>[4x]HHHHHHMALQLAAHSDARSGPVGSNGGQFWSFRPVRPLNKIVLSFSGSPDQTLNLISITFSSNPTDIITVGGVGPEPLTYTETVNIDGDIIEISGMIANYKGYNVIRSIKFTTNKKEYGPYGANAGTPFNIKIPDGNKIVGFFGNSGWYVDAIGAYYTAK

Structural and functional analysis identified IPO as a member of the JRL family but with a different tetrameric association. The monomeric IPO from residues 1 to 154 shows a typical β-prism fold found in the JRL family, with 12 β-sheets (β3-β14) and 2 additional short, extended, N-terminal β-strands (β1-β2). Four IPO protomers form a compact tetrameric association by swapping their extended N termini from residues 1 to 10. Thus, the wound-inducible protein IPO from sweet potato has versatile carbohydrate binding properties and might play a role in plant defense.

IPO–Me-Gal belongs to an orthorhombic space group P212121. The Matthews coefficient and solvent content were 2.25 Å3/Da and 45.2%, respectively, for 4 molecules in an asymmetric unit. The 4 IPO–Me-Gal molecules shown in Figure 1D form the same tetrameric association as that of IPO–Me-Glc. In the structure IPO–Me-Gal, 10 hydrogen bonds are formed by the same residues Gly21, Tyr97, Gly141, Trp142, Tyr143, and Asp145 of IPO. The atom C7 of Me-Gal is shown in the Me…π interaction with Trp142 of IPO. However, Me-Gal and Me-Glc are epimers at the C4 position. The C4 atom of Me-Glc and Me-Gal could form one hydrogen bond with the amine group of Gly21 of IPO and one hydrogen bond with the β-carboxylic group of Asp145 of IPO. The KA values for Me-Gal and Me-Glc were 4.09×103 M−1 and 2.01×103 M−1, respectively.> GPLGSMEELTLTILRQTGGLGISIAGGKGSTPYKGDDEGIFISRVSEEGPAARAGVRVGDKLLEVNGVALQGAEHHEAVEALRG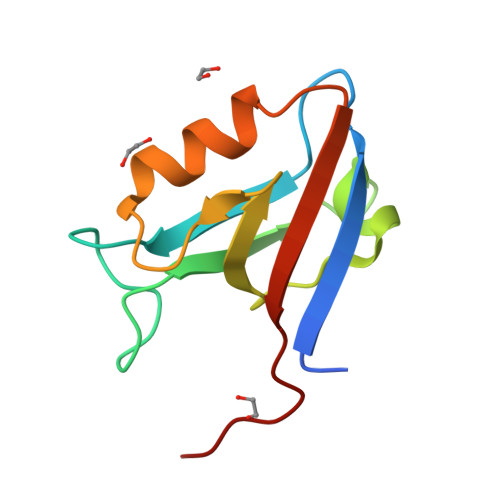AGTAVQMRVWRERETSV>FQSITSPAKAVAKQENVVQLASEQPKVEMNKTAPSRFNGKERKVAYLTFDDGPGKYTAELLNTLKQHDAKATFFLIGANVKEFPDLVKRENAEGHYVGMHSMTHNFAKLYKNGEYVNEMKEDQGLIANIIGKSPKLTRPPYGSMPGLNEGLRNKVVEGGFKVWDWTIDSLDWRYNKMPVDAAAAQIAQNVLTNATKPQEVILMH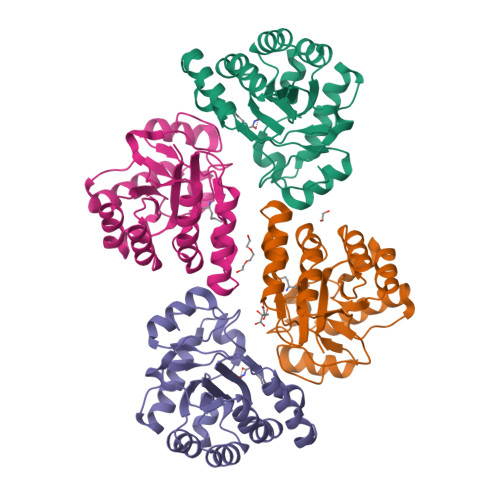DIHPQSVAAVPAILKGLKEKGYEFEAYHEESHFPVNFWHDNRM[4x]> GGGAAGAUACAAGGUGAGCCCAAUAAUAUGGUUUGGGUU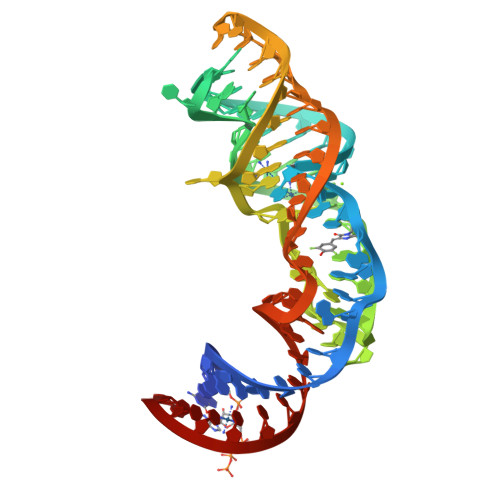AGGAUAGGAAGUAGAGCCUUAAACUCUCUAAGCGGUAUCUUCCC>EQARPADDALAALGAQLFVDPALSRNATQSCATCHDPARAFTDPREGKAGLAVSVGDDGQSHGDRNTPTLGYAALVPAFHRDANGKYKGGQFWDGRADDLKQQAGQCMLNPVEMAMPDRAAVAARLRDDPAYRTGFEALFGKGVLDDPERAFDAAAEALAAYQATGEFSPFDSKYDRVMRGEEKFTPLEEFGYTVFITWNCRLCHMQRKQGVAERETFTNFEYHNIGLPVNETAREASGLGADHVDHGLLARPGIEDPAQSGRFKVPSLRNVAVTGPYMHNGVFTDLRTAILFYNKYTSRRPEAKINPETGAPWGEPEVARNLSLAELQSGLMLDDGRVDALVAFLETLTDRRYEPLLEESRAAQKDHHHHHH[2x];>[2x]ADAPAGTDPRAKWVPQDNDIQACDYWRHCSIDGNICDCSGGSLTNCPPGTKLATASWVASCYNPTDGQSYLIAYRDCCGYNVSGRCPCLNTEGELPVYRPEFANDIIWCFGAEDDAMTYHCTISPIVGKASHHHHHH;>[2x]DAPEAETQAQETQGQAAARAAAADLAAGQDDEPRILEAPAPDARRVYVNDPAHFAAVTQQFVIDGEAGRVIGMIDGGFLPNPVVADDGSFIAHASTVFSRIARGERTDYVEVFDPVTLLPTADIELPDAPRFLVGTYPWMTSLTPDGKTLLFYQFSPAPAVGVVDLEGKAFKRMLDVPDCYHIFPTAPDTFFMHCRDGSLAKVAFGTEGTPEITHTEVFHPEDEFLINHPAYSQKAGRLVWPTYTGKIHQIDLSSGDAKFLPAVEALTEAERADGWRPGGWQQVAYHRALDRIYLLVDQRDEWRHKTASRFVVVLDAKTGERLAK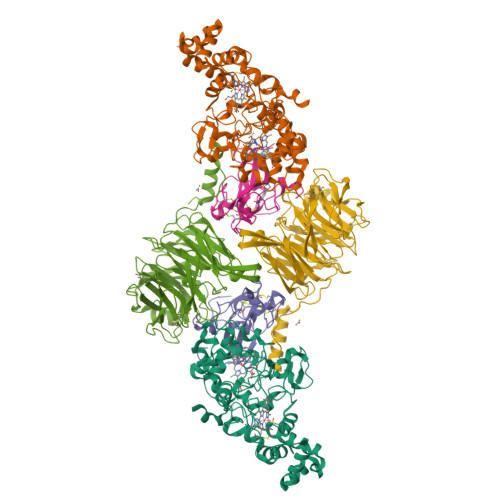FEMGHEIDSINVSQDEKPLLYALSTGDKTLYIHDAESGEELRSVNQLGHGPQVITTADMG> GSSPQREPQRVSHEQFRAALQLVVDPGDPRSYLDNFIKIGEGSTGIVCIATVRSSGKLVAVKKMDLRKQQRRELL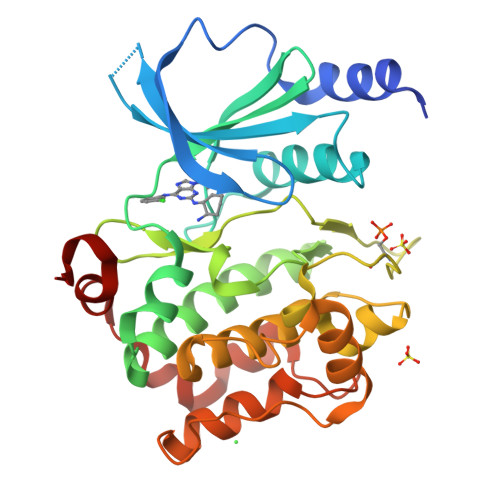FNEVVIMRDYQHENVVEMYNSYLVGDELWVVMEFLEGGALTDIVTHTRMNEEQIAAVCLAVLQALSVLHAQGVIHRDIKSDSILLTHDGRVKLSDFGFCAQVSKEVPRRKSLVGTPYWMAPELISRLPYGPEVDIWSLGIMVIEMVDGEPPYFNEPPLKAMKMIRDNLPPRLKNLHKVSPSLKGFLDRLLVRDPAQRATAAELLKHPFLAKAGPPASIVPLMRQNRTR In this pathway, adenylosuccinate lyase (PurB; EC 4.3.2.2) catalyzes the breakdown of 5-aminoimidazole-4-(N-succinylcarboxamide) ribotide (SAICAR) to 5-aminoimidazole-4-carboxamide ribotide (AICAR) and fumarate. PurB demonstrates dual substrate specificity and can also break down adenylo­succinate to adenosine monophosphate (AMP) and fumarate; therefore, it also determines the levels of AMP and fumarate in the cell via the purine-nucleotide cycle. PurB is classified along with arginosuccinate lyase, l-­aspartase, class II fumarases and 3-carboxymuconate lactonase as a member of the aspartase/fumarase or β-elimination superfamily of enzymes. PurB catalyzes a β-elimination that is thought to occur via a general acid–base uni–bi mechanism.

We describe the construction of an efficient bacterial recombinant expression system, enzyme purification and crystallization protocols and report the crystal structure of PurB from S. aureus (SaPurB) at 2.5 Å resolution. Our structure contains one of the reaction products, AMP, bound in the active site and a nearby strong feature of electron density has been modelled and successfully refined as oxalate. The SaPurB subunit can be divided into three domains that combine to form an elongated structure. As will be described, SaPurB forms a tetramer in the crystal structure and this rules out space group I212121. The tetramer contains four active sites, each formed by regions donated from three different subunits. The AMP phosphate accepts hydrogen bonds from Arg4C, Tyr5C, Asn276C, Ser306A, Arg310A and via a water-mediated association with Arg326A. The adenine N1 accepts a hydrogen bond from Thr95A OG1; N6 donates hydrogen bonds to His141B NE2 and Gln212A OE1, residues which are themselves positioned by hydrogen-bonding interactions. His141 in SaPurB corresponds to His171 in E. coli PurB and is the catalytic acid for the mechanism. The oxalate binds accepting hydrogen bonds donated from Ser94A OG and Gln259A NE2 and a water molecule that in turn interacts with the side chain of Thr95. One side of the SaPurB active site is formed by a mobile loop that links β5 and α12.

> MIERYSREEMSNIWTDQNRYEAWLEVEILACEAWSELGHIPKADVQKIRQNAKVNVERAQEIEQETRHDVVAFTRQVSETLGEERKWVHYGLTSTDVVDTALSFVIKQANDIIEKDLERFIDVLAEKAKNYKYTLMMGRTHGVHAEPTTFGVKMALWYTEMQRNLQRFKQVREEIEVGKMSGAVGTFANIPPEIESYVCKHLGIGTAPVSTQTLQRDRHAYYIATLALIATSLEKFAVEIRNLQKTETREVEEAFAKGQKGSSAMPHKRNPIGSENITGISRVIRGYITTAYENVPLWHERDISHSSAERIMLPDVTIALDYALNRFTNIVDRLTVFEDNMRNNIDKTFGLIFSQRVLLALINKGMVREEAYDKVQPKAMISWETKTPFRELIEQDESITSVLTKEELDECFDPKHHLNQVDTIFERAGLA> GHMTLPTKTSTLDVAAQCFLNSLVRETKDWRLTEYQPTQLIIPLGEQQALHFRVAYFSPTQHHRFEF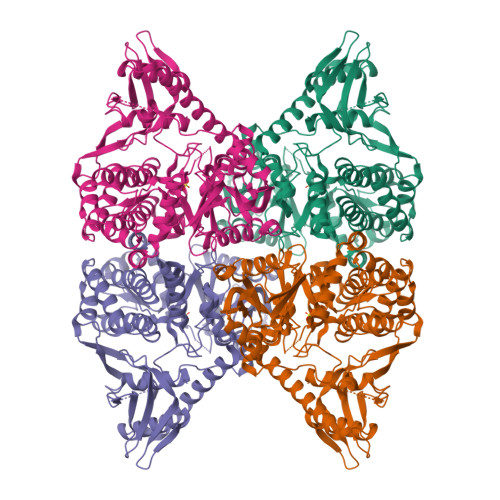PARLVTASGSHPVDFATLSRLIVDKLQHQLLLPATSCETFHQRVMESHAHTQQAIDARHDWAALREKALNFGEAEQALLVGHAFHPAPKSHEPFNQQEAERYLPDFAPHFPLRWFAVNKTQIAGESLHLNLQQRLTRFAAENAPQLLNELSDNQWLFPLHPWQGEYLLQQEWCQELVAKGLIKDLGEAGAPWLPTTSSRSLYCATSRDMIKFSLSVRLTNSVRTLSVKEVKRGMRLARLAQTDDWQTLQARFPTFRVMQEDGWAGLRDLHGNIMQESLFALRENLLVDQPQSQTNVLVSLTQAAPDGGDSLLVAAVKRLSDRLGITAQQAAHAWVDAYCHQVLKPLFTAEADYGLVLLAHQQNILVQMLGDLPVGLIYRDCQGSAFMPHAAGWLDTIGEAQAENVFTREQLLRYFPYYLLVNSTFAVTAALGAAGLDSEANLMARVRTLLAEMRDQVTHKTCLNYVLENPYWNVKGNFFCYLNDHNENTIVDPSVIYFDFANPLLAQEG(1R)-1-cyclopentyl-2,2,2-trifluoroethyl 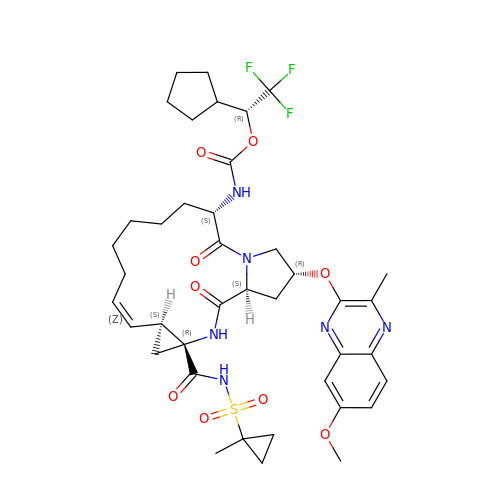{(2R,4R,6S,12Z,13aS,14aR,16aS)-2-[(7-methoxy-3-methylquinoxalin-2-yl)oxy]-14a-[(1-methylcyclopropane-1-sulfonyl)carbamoyl]-5,16-dioxo-1,2,3,5,6,7,8,9,10,11,13a,14,14a,15,16,16a-hexadecahydrocyclopropa[e]pyrrolo[1,2-a][1,4]diazacyclopentadecin-6-yl}carbamate | C40 H51 F3 N6 O9 S | NIVLDUFKSNQSFW-FKWQUPSWSA-N>IEEEDVICDGCNGPVVGTRYKCSVCPDYDLCSVCEGKGLHRGHTKLAFPSPFGHLSEGFS[2x]

Intriguingly, the autophagy adapter p62/SQSTM1/Sequestosome-1 was recently reported to recognize N-degrons, the N-end rule substrates of the well-characterized UPS, and where ultimately these substrates are delivered to ALS8,9. p62 is a key selective autophagy adapter that plays a role in the degradation of various cellular constituents such as misfolded proteins and their aggregates, malfunctioning organelles, and invading pathogens. Intriguingly, it was recently reported that the central ZZ-domain in p62 plays a critical role in the recognition of N-terminal arginylated BiP/GRP78 by the Arg-tRNA transferase ATE1. Here, we present the high resolution structures of the ZZ-domain of p62 in complex with 8 different N-degrons including type-1 and type-2, and subsequently identify key determinants involved in the unusual recognition.

However, an understanding of the manner by which the ZZ-domain binds to type-2 substrates is problematic since there is no deep hydrophobic pocket in the ZZ-domain, which is known to be involved in the recognition mode for type-2 N-degrons. Therefore, we determined the structure of the ZZ-domain in complex with a variety of N-degrons comprising three type-1 N-degrons and five type-2 N-degrons. As described for the R-BiP complex, two aspartic acid residues, Asp129 and Asp149, bind to the α-amino group, and Asp147 forms a hydrogen bond with the first peptide bond, which means that these interactions are conserved in all different N-terminal residues. However, the side chain of the N-terminal residue of the N-degron is recognized differently. Furthermore, the hydrophobic side chain of Ile127 guides the orientation of the side chain of the primary residue. Therefore, relatively small and branched hydrophobic residues at the primary position might provide very weak (or no) interactions with the binding patch of the ZZ-domain.> GAGEVKKATAEEVHARIEFLWQREQEKKKEQVV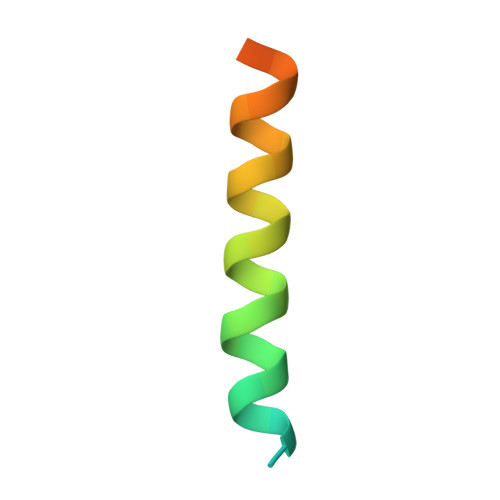SLK> MKDLVDTTEMYLRTIYELEEEGVTPLRARIAERLEQSGPTVSQTVARMERDGLVVVASDRSLQMTPTGRTLATAVMRKHRLA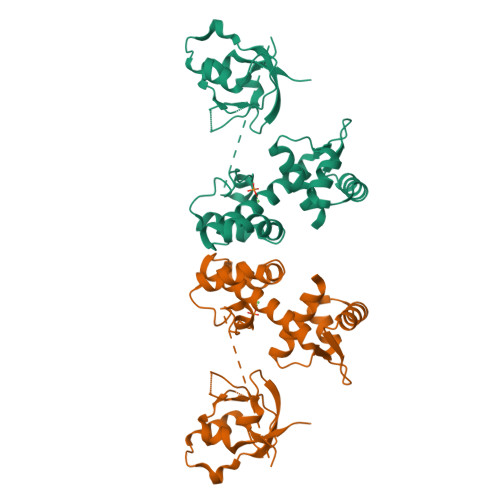ERLLTDIIGLDINKVHDEACRWEHVMSDEVERRLVKVLKDVSRSPFGNPIPGLDELGVGNSDAAVPGTRVIDAATSMPRKVRIVQINEIFQVKTDQFTQLLDADIRVGSEVEIVDRDGHITLSHNGKDVELLDDLAHTIRIEEL>[12x]GSHMAKYTKEDIFRFADEQNVKFIRLQFTDILGIIKNVEIPVSQLKKALDNKIMFDGSSIEGFVRIEESDMYLFPDLDTWVVFPWTAEKGKVARMICDIYNPDMTPFAGDPRANLKRVLKEMEELGFTEFNLGPEPEFFLFKLDENRRPTLELNDSGGYFDLAPTDLGENCRRDIVLELEEMGFEIEASHHEVAPGQHEIDFKYEDAITACDSIQ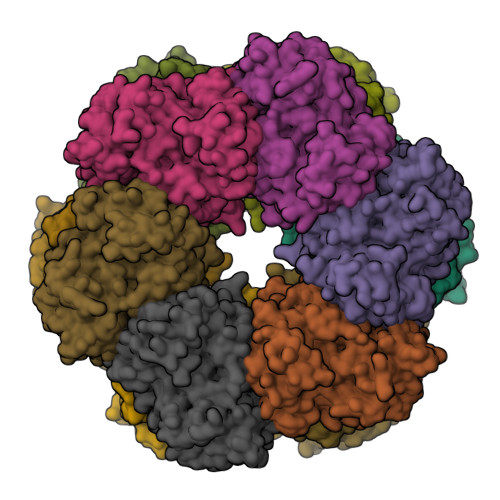TFKLVVKTIARKHGLHATFMPKPLFGVNGSGMHFNMSLFNEKGNAFFDESGELELSQTAYHFLAGMLKHARGYTAVTNPTINSFKRLVPGYEAPCYIAWSGKNRSPLVRVPSSRGLSTRLELRSVDPSANPYLAMAVLLKAGLSGIKDELTPPAPVDRNIYGMNEEEREATGIYDLPESLGHALIELEKNEIIKDGLGEHIFEHFIEAKTIECDMFRTAVHPWEREQYLEIY>MSLEKLKLIGDERLDYLLAENLRIIQSPSVFSFSIDAVLLAKFSYLPIRKGKIIDLCSGNGIIP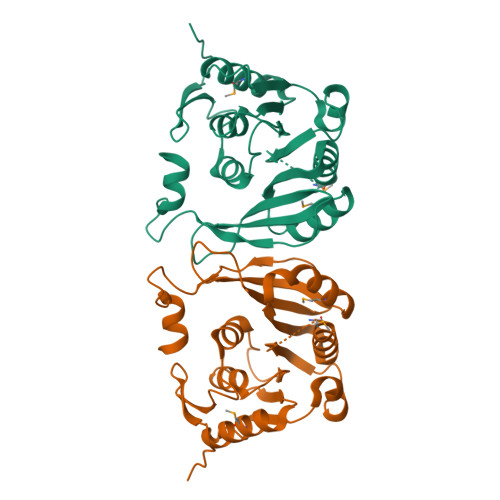LLLSTRTKAKIVGVEIQERLADMAKRSVAYNQLEDQIEIIEYDLKKITDLIPKERADIVTCNPPYFATPDTSLKNTNEHFRIARHEVMCTLEDTIRVAASLLKQGGKANFVHRPERLLDIIDIMRKYRLEPKRIQFVHPRSDREANTVLVEGIKDGKPGVKYVPPVIVYDELGEYTPVIKEILYGESEGHHHHHH[2x]>MPTSNPAKPLDGFRVLDFTQNVAGPLAGQVLVDLGAEVIKVEAPGGEAARQITSVLPGRPPLATYFLPNNRGKKSVTVDLTTEQAKQQMLRLADTADVVLEAFRPGTMEKLGLGPDDLRSRNPNLIYARLTAYGGNGPHGSRPGIDLVVAAEAGMTTGMPTPEGKPQIIPFQLVDNASGHVLAQAVLAALLHRERNGVADVVQVAMYDVAVGLQANQLMMHLNRAASDQPKPEPAPKAKRRKGVGFATQPSDAFRTADGYIVISAYVPKHWQKLCYLI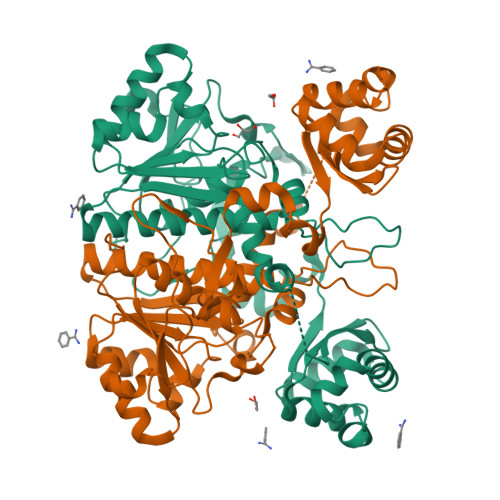GRPDLVEDQRFAEQRSRSINYAELTAELELALASKTATEWVQLLQANGLMACLAHTWKQVVDTPLFAENDLTLEVGRGADTITVIRTPARYASFRAVVTDPPPTAGEHNAVFLARP[4x]> MMKMRWLSAAVMLTLYTSSSWAFSIDDVAKQAQSLAGKGYETPKSNLPSVFRDMKYADYQQIQFNHDKAYWNNLKTPFKLEFYHQGMYFDTPVKINEVTATAVKRIKYSPDYFTFGDVQHDKDTVKDLGFAGFKVLYPINSKDKNDEIVSMLGASYFRVIGAGQVYGLSARGLAIDTALPSGEEFPRFKEFWIERPKPTDKRLTIYALLDSPRATGAYKFVVMPGRDTVVDVQSKIYLRDKVGKLGVAPLTSMFLFGPNQPSPANNYRPELHDSNGLSIHAGNGEWIWRPLNNPKHLAVSSFSMENPQGFGLLQRGRDFSRFEDLDDRYDLRPSAWVTPKGEWGKGSVELVEIPTNDETNNNIVAYWTPDQLPEPGKEMNFKYTITFSRDEDKLHAPDNAWVQQTRRSTGDVKQSNLIRQPDGTIAFVVDFTGAEMKKLPEDTPVTAQTSIGDNGEIVESTVRYNPVTKGWRLVMRVKVKDAKKTTEMRAALVNADQTLSETWSYQLPANELEHHHHHH

Most Gram-negative bacteria synthesize osmo-regulated periplasmic glucans (OPG) in the periplasm or extracellular space. In this study, structural and functional analyses of OpgG and OpgD from Escherichia coli revealed that these proteins are β-1,2-glucanases with remarkably different activity from each other, establishing a new glycoside hydrolase family, GH186. Furthermore, a reaction mechanism with an unprecedentedly long proton transfer pathway among glycoside hydrolase families is proposed for OpgD. The conformation of the region that forms the reaction pathway differs noticeably between OpgG and OpgD, which explains the observed low activity of OpgG.

To generate hypotheses regarding the very low reaction velocities of EcOpgG, we determined the complex structure of EcOpgG (D361N mutant) with β-1,2-glucan at 1.81 Å resolution. In the catalytic pocket of the complex, the electron density of a Sop16 molecule was observed. The dynamic conformational change from a loop (residues 409–425) to two β-strands upon substrate binding is a unique feature found in EcOpgG. However, the β-sheet interacts not with the substrate but with the α-helix 3 in the complex. The motion of α-helix 3 is induced by the interactions between Y56 in the helix and the 6-hydroxy group of the Glc moiety. These observations suggest that the closure motion of α-helix 3 is required for forming the β-sheet. A β-1,2-glucan molecule binds to the substrate pocket in the complex of EcOpgG at almost the same position as EcOpgD, except at the subsites –5 to –7 in EcOpgD. The only Glc moiety forming 1S3 in EcOpgG is the well-superimposed Glc moiety at subsite –1 in EcOpgD. However, electron density for nucleophilic water is poor in EcOpgG, which strongly supports the observed low SGL activity of EcOpgG. However, the absence of a nucleophilic water molecule and the presence of a branched proton transfer pathway from Wat2 may be responsible for the low specific activity of EcOpgG (0.11 U/mg).> EDVVWRWSCDNGKCVKLKNDPRSSEPALSLEACKMFCNEYGLLWPRPTGEADLGNFLSKINLNSIEVKILKKGATDDLMEAAAKRFKEQVSLAIPRGSTPKLTGKAVDVYLVNENPNEKAFSLEMDESYGLRVSPSGADRVNATITANSFFGMRHGLETLSQLFVFDDIRDHLLMVRDVNISDKPVYPYRGILLDTARNYYSIESIKRTIEAMAAVKLNTLHWH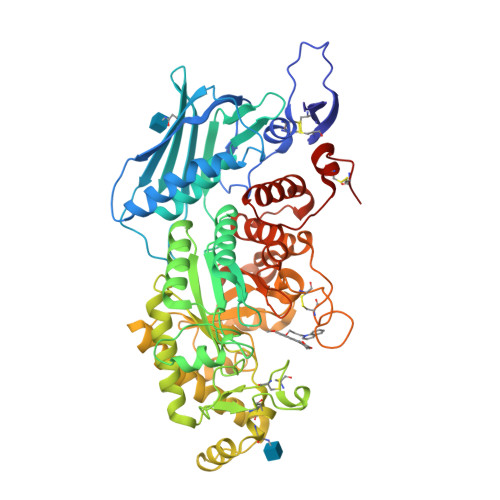ITDSQSFPFVTTKRPNLYKFGALSPQKVYTKAAIREVVRFGLERGVRVLPEFDAPAHVGEGWQDTDLTVCFKAEPWKSYCVEPPCGQLNPTKDELYQYLEDIYSDMAEVFDTTDIFHMGGDEVSEACWNSSDSIQNFMMQNRWDLDKESFLKLWNYFQQKAQDKAYKAFGKKLPLILWTSTLTNYKHIDDYLNKDDYIIQVWTTGVDPQIKGLLEKGYRLIMSNYDALYFDCGYGAWVGAGNNWCSPYIGWQKVYDNSPAVIALEHRDQVLGGEAALWSEQSDTSTLDGRLWPRAAALAERLWAEPATSWQDAEYRMLHIRERFVRMGIQAESLQPEWCYQNEGYCYSHHHHHH> MAGLELLSDQGYRVDGRRAGELRKIQARMGVFAQADGSAYIEQGNTKALAVVYGPHEIRGSRARALPDRALVNCQYSSATFSTGERKRRPHGDRKSCEMGLQLRQTFEAAILTQLHPRSQIDIYVQVLQADGGTYAACVNAATLAVLDAGIPMRDFVCACSAGFVDGTAL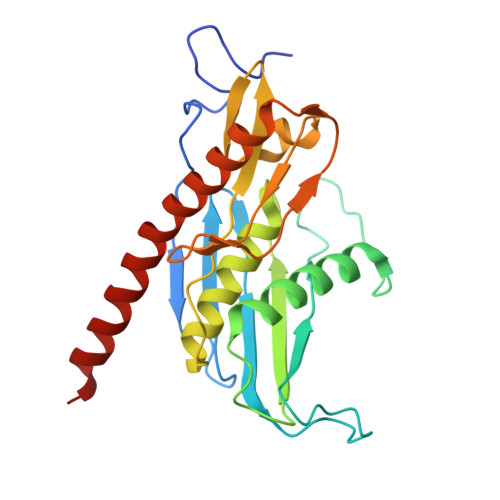ADLSHVEEAAGGPQLALALLPASGQIALLEMDARLHEDHLERVLEAAAQAARDVHTLLDRVVRQHVREASILLGD> GPMAAEEEDEVEWVVESIA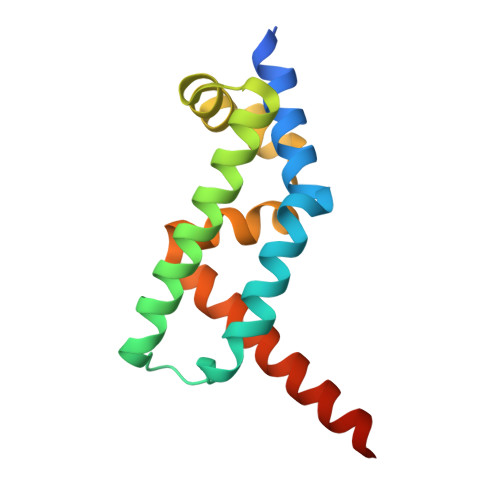GFLRGPDWSIPILDFVEQKCEVFDDEEESKLTYTEIHQEYKELVEKLLESYLKEIGINEDQFQEACTSPLAKTRTSQAILQPVLAAEDFTIFKAMMVQKNIEMQLQAIRIIQERNG>[3x]MNKILLVDDDRELTSLLKEL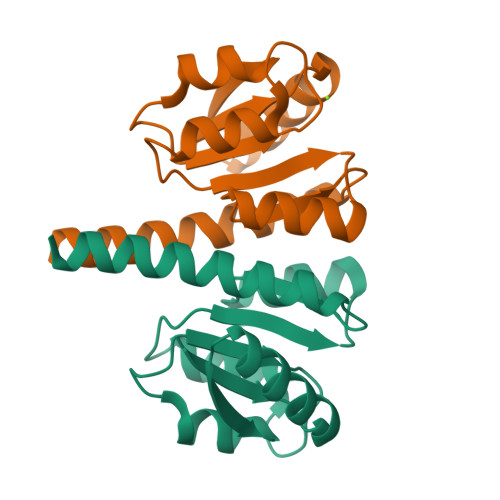LEMEGFNVIVAHDGEQALDLLDDSIDLLLLDVMMPKKNGIDTLKALRQTHQTPVIMLTARGSELDRVLGLELGADDYLPKPFNDRELVARIRAILRRSHWSEQKLAAALEHHHHHH6-ethoxy-2-methyl-1,3-benzothiazole 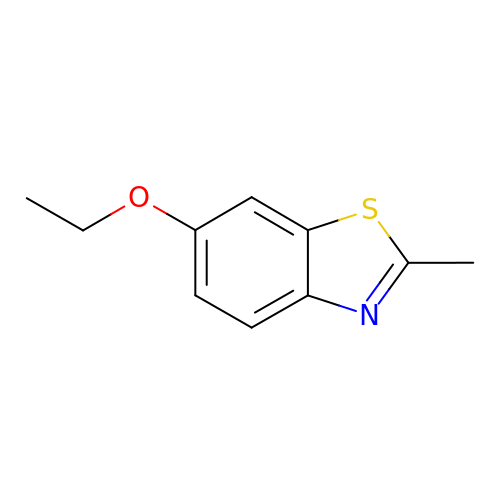| C10 H11 N O S | PKRZJVQWLOOWHD-UHFFFAOYSA-N> DSLGREAKCYNELNGCTYE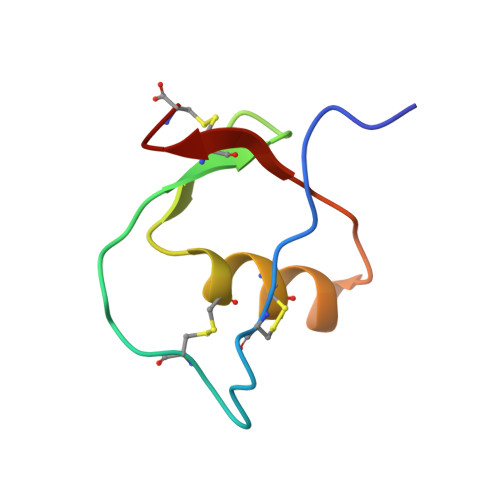YRPVCGTDGDTYPNECVLCFENRKRQTSILIQKSGPC> MAHHHHHHLPALKLALEYIVPCMNKHGICVVDDFLGKETGQQIGDEVRALHDTGKFTDGQLVSQKSDSSKDIRGDKITWIEGKEPGCETIGLLMSSMDDLIRHCNGKLGSYKINGRTKAMVACYPGNGTGYVRHVDNPNGDGRCVTCIYYLNKDWDAKVSGGILRIFPEGKAQFADIEPKFDRLLFFWSDRRNPHE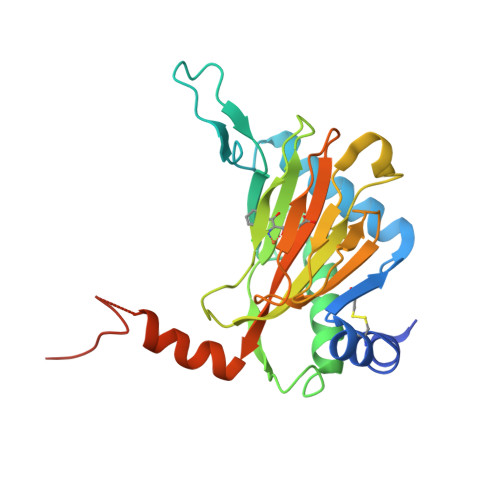VQPAYATRYAITVWYFDADERARAKVKYLTGEKGVRVELNKPSDSVGKDVF(7R)-4,7-DIHYDROXY-N,N,N-TRIMETHYL-10-OXO-3,5,9-TRIOXA-4-PHOSPHAHEPTACOSAN-1-AMINIUM 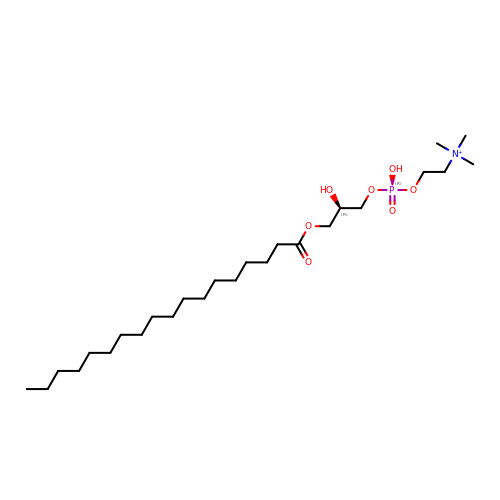4-OXIDE | C26 H55 N O7 P | IHNKQIMGVNPMTC-RUZDIDTESA-O> CVNI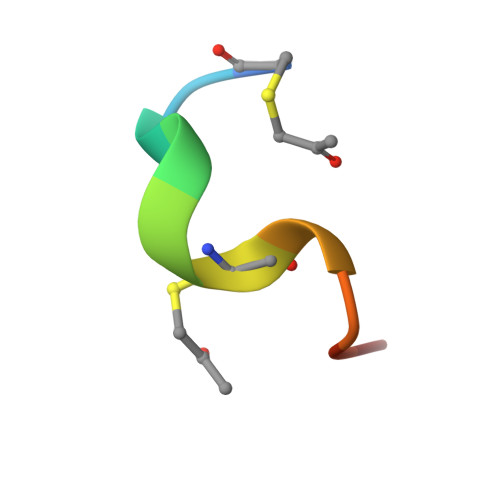MCCRCPX> K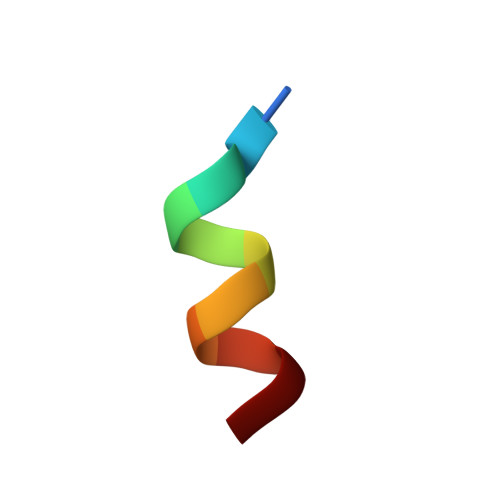HKILHRLLQD>[2x]GSHMASNDLIYQDEHASLQPLEGRTVAVIGYGIQGR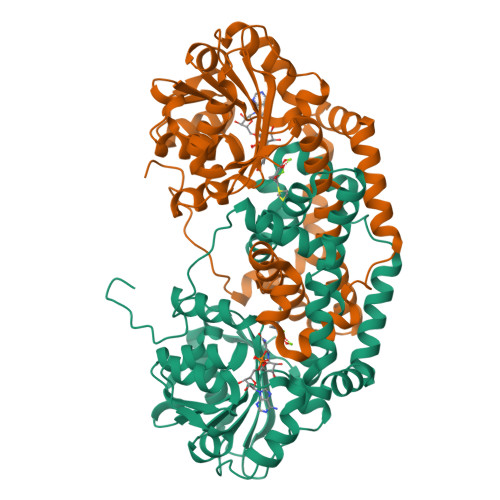AFAANLRDSGVAVRVGNIDDRYFELARAEGHRVTNIAEAVAHADIVLLLIPDEAHGAVFDVDIAPNLRDGALLCVAHGHSLVQGDVRPLPGRDLAMLAPRMYGDPIRRYYLAGQGAPAYFDIVADHTGRARDRVLAIARAVGFTRAGVMALGYRQETFLDLFQEQFLAPALVDLVETGFQVLVERGFNPKAALLEVYGSGEMGKMMLDGADIGLDEVVALQGSPTCQVGYHRWRGRTLPTAVRELAARVLDQIEGGDFSAYLKEQASNDYASLDDARRAALKRPLNVAHAQVRAAFRFPTEAAGGLYQAAQAPADVEPEAAR> MDETVAEFIKRTILKIPMNELTTILKAWDFLSENQLQTVNFRQRKESVVQHLIHLCEEKRASISDAALLDIIYMQFHQHQKVWDVFQMSKGPGEDVDLFDMKQFKNSFKKILQRALKNVTVSFRETEENAVWIRIAWGTQYTKPNQYKPTYVVYYSQTPYAFTSSSMLRRNTPLLGQALTIASKHHQIVKMDLRSRYLDSLKAIVFKQYNQTFETHNSTTPLQERSLGLDINMDSRIIHENIVEKERVQRITQETFGDYPQPQLEFAQYKLETKFKSGLNGSILAEREEPLRCLIKFSSPHLLEALKSLAPAGIADAPLSPLLTCIPNKRMNYFKIRD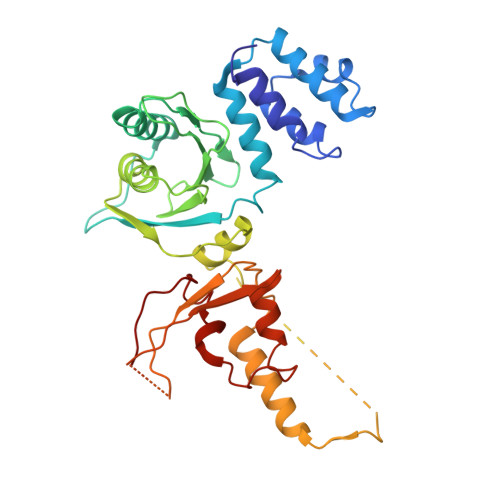K>VNFPNIPAEGVQFRLRARDTGYVIYSRTENPPLVWQYNGPPYDDQLFTLIYGTGPRKNLYAIKSVPNGRVLFSRTSASPYVGNIAGDGTYNDNWFQFIQDDNDPNSFRIYNLASDTVLYSRTTADPKFGNFTGAKYDDQLWH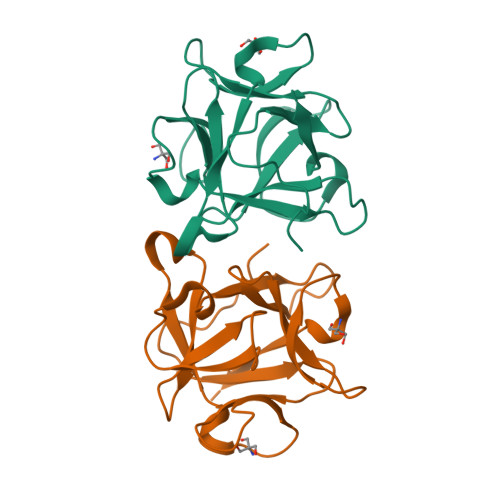FELV[4x]>[2x]SKITYTFTDEAPALATYSLLPIVKAFAASAGIDVETSDISLAGRILANFADRLEADQRIEDDLARLAVLATSPDANIIKLPNISASVPQLKGAIAELQGLGYKVPDFPEDPQTDEEKEVRARYAKILGSAVNPVLREGNSDRRAPAAVKAYARKHPHSMGKWSMASRSHADYMRGGDFFSSEQSITMAKAGDVRIEFVGKD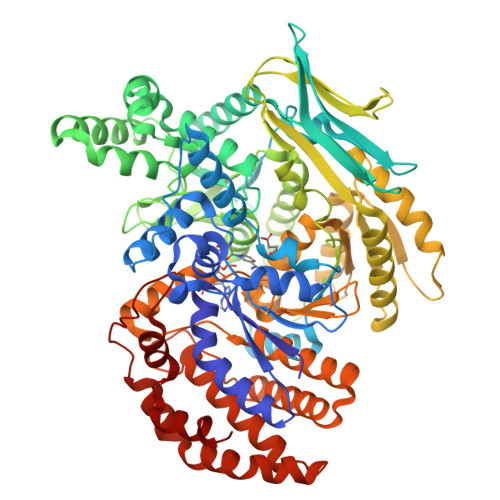GKVEVKKQLSLQEGEVLDSMFMSCGKLRDFFEKTLQDCKETGVMWSLHVKATMMKISHPIVFGHAVSVYYKDVFDKWGQLFEELGVNPNNGISSVYDKIKSLPASQQEEILHDIHEVYSHRPEMAMVDSVKGITNLHIPSDVIVDASMPAMIRNSGQMWGKDGKQKDTKAVMPESTYARIYQEMINFCKTNGAFDPTTMGSVPNVGLMAQKAEEYGSHDKTFEMTADGTMRVVLADGSVLMQHKVETGDIWRACQTKDAPIRDWVKLAVTRARQSDTPAIFWLDPERAHDRELRKKVELYLKDHDLTGLDISIMGYNEAIRVSMERLIRGKDTISVTGNVLRDYLTDLFPIMELGTSAKMLSIVPLMAGGGMYETGAGGSAPKHVQQLVEENYLRWDSLGEFLALAVSLEETGIKTGNAKAKLLGKALDEATGKLLDNNKSPSRKVGDIDNRGSHFYLAMYWAQALAAQNEDAELKAHFAPLAKALTEQEATIVAELNAVQGKPAEIGGYYRSNPELTSKVMRPSATFNAAIDSLA>[2x]MHHHHHAIYNVEVETGDREHAGTDATITIRITGAKGRTDYLKLDKWFHNDFEAGSKEQYTVQGFDVGDIQLIELHSDGGGYWSGDPDWFVNRVIIISSTQDRVYSFPCFRWVIKDMVLFPGEATLPFNEVPAIVSEQRQKELEQRKLTYQWDYVSDDMPGNIKAKTHDDLPRDVQFTDEKSRSYQESRKAALVNLGIGSLFTMFENWDSYDDYHILYRNWILGGTPNMADRWHEDRWFGYQFLNGANPVILTRCDALPSNFPVTNEHVNASLDRGKNLDEEIKDGHIYIVDFKVLVGAKSYGGPVLEDIGYKVPDHLKHDEADIRYCAAPLALFYVNKLGHLMPIAIQINQEPGPENPIWTPHEENEHDWMMAKFWLGVAESNFHQLNTHLLRTHLTTESFALSTWRNLASAHPVFKLLQPHIYGVLA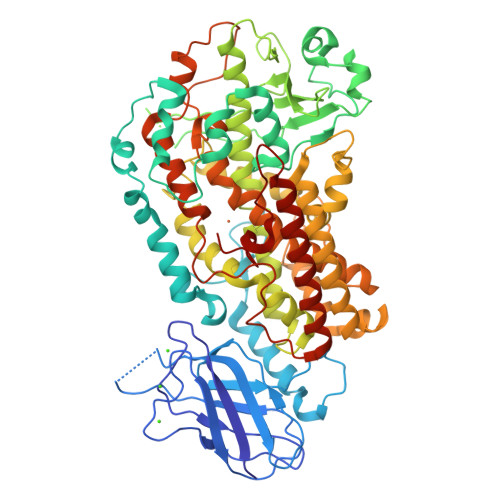IDTIGRKELIGSGGIVDQSLSLGGGGHVTFMEKCFKEVNLQDYHLPNALKKRGVDDPSKLPGFYYRDDGLALWEAIETFIGEIIAIFYKNDDDVKRDNEIQSWIYDVHKNGWRVNPGHQDHGVPASFESREQLKEVLTSLVFTFSCQHAAVNFSQKDHYGFTPNAPAVLRHPPPKKKGEATLQSILSTLPSKSQAAKAIATVYILTKFSEDERYLGNYSATAWEDKDALDAINRFQDKLEDISKKIKQRNENLEVPYIYLLPERIPNGTAI>[4x]MSTAEPAPDPTNPSTSGLAPTTNGIGSPPPTASAATKFSILTKFLRRKNQVHTTTAQQNEFMQKYMPNGNSNAVQPAATGGQPASSDGGSAIEVPPPKESYAVRIRKYLANYTQDPSTDNFYYWTCVVTVAYIYNLLFVIARQVFNDLIG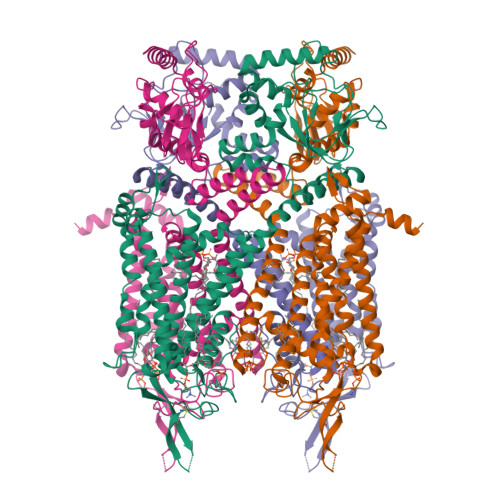PSSQSLCRFYNGTLNSTTQVECTYNMLTNMKEMPTYSQYPDLGWSKYWHFRMLWVFFDLLMDCVYLIDTFLNYRMGYMDQGLVVREAEKVTKAYWQSKQYRIDGISLIPLDYILGWPIPYINWRGLPILRLNRLIRYKRVRNCLERTETRSSMPNAFRVVVVVWYIVIIIHWNACLYFWISEWIGLGTDAWVYGHLNKQSLPDDITDTLLRRYVYSFYWSTLILTTIGEVPSPVRNIEYAFVTLDLMCGVLIVATIAGNVGSMISNMSAARTEFQNKMDGIKQYMELRKVSKQLEIRVIKWFDYLWTNKQSLSDQQVLKVLPDKLQAEIAMQVHFETLRKVRIFQDCEAGLLAELVLKLQLQVFSPGDFICKKGDIGREMYIVKRGRLQVVDDDGKKVFVTLQEGSVFGELSILNIAGSKNGNRRTANVRSVGYTDLFVLSKTDLWNALREYPDARKLLLAKGREILKKDNLLDENAPEEQKTVEEIAEHLNNAVKVLQTRMARLIVEHSSTEGKLMKRIEMLEKHLSRYKALARRQKTMHGVSIDGGDISTDGVDERVRPPRLRQTKTIDLPTGTESESLLK3-{(E)-[(3-{[(2,6-dioxo-1,2,3,6-tetrahydropyrimidin-4-yl)methyl]amino}propoxy)imino]methyl}benzoic 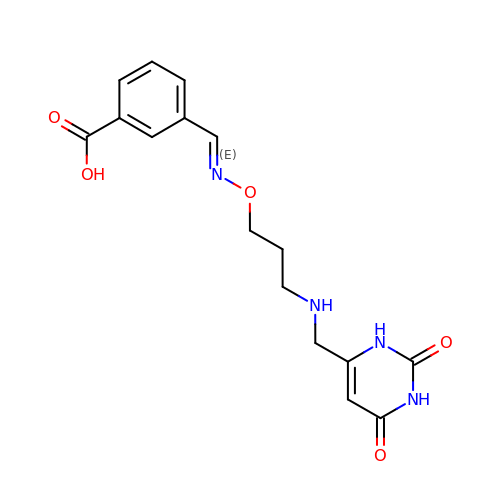acid | C16 H18 N4 O5 | DNNMFLCWPRQYIC-GIJQJNRQSA-N7-[[5-[(methylideneamino)methyl]pyridin-3-yl]oxymethyl]quinolin-2-amine 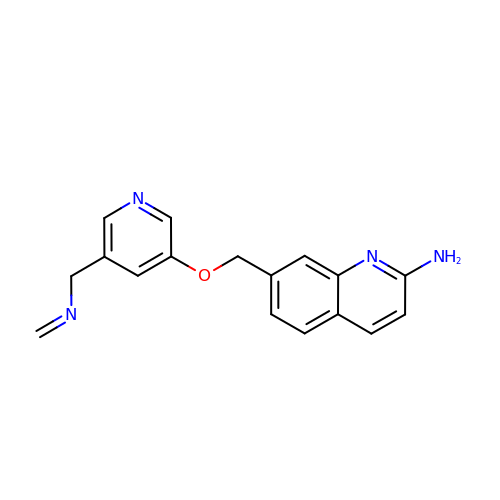| C17 H16 N4 O | JWSPKIZRSASLMF-UHFFFAOYSA-N>GSPEFSGREAKSRRRTSLPAPSPSSSNISLWNILRNNIGKDLSKVAMPVELNEPLNTLQRLCEELEYSELLDKAAQIPSPLERMVYVAAFAISAYASSYYRAGSKPFNPVLGETYECIREDKGFQFFSEQVSHHPPISACHAESRNFVFWQDVRWKNKFWGKSMEIVPIGTTHVTLPVFGDHFEWNKVTSCIHNILSGQRWIEHYGEIVIKNLHDDSCYCKVNFIKAKYWSTNAHEIEGTVFDRSGKAVHRLFGKWHESIYCGGGSSS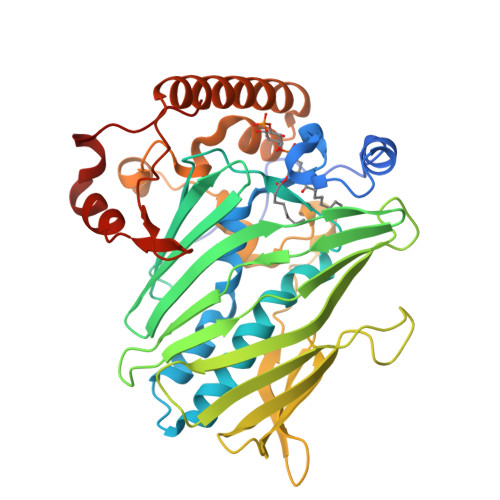ACVWRANPMPKGYEQYYSFTQFALELNEMDPSSKSLLPPTDTRFRPDQRFLEEGNLEEAEIQKQRIEQLQRERRRVLEENHVEHQPRFFRKSDGSWVSNGTYLELRKDLGFSKLDHPVLW[2x]2,3,4,5,6-pentafluoro-N-hydroxybenzamide | C7 H2 F5 N O2 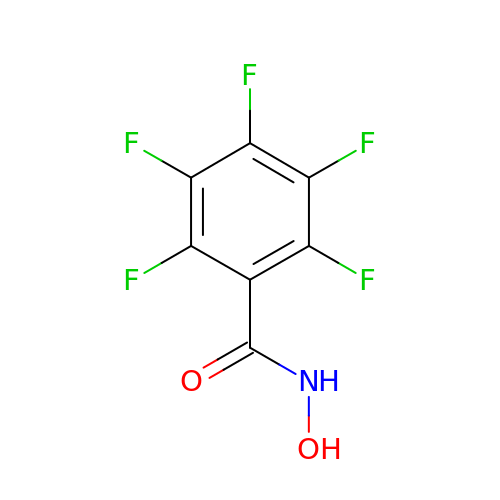| MANBOMDQSILBJG-UHFFFAOYSA-N>[4x]GIDPFTMTPSEDFVVTDRGGIVENSHRVHAAVVDAKGRLLYALGNPTRMTLARSAAKPAQALAILETEGVAGYGFDDADIALMCASHSSEDRHIARTRAMLSKIKAEEADLRCGGHPSLSEMVNRSWIKQDFIPTAVCSNCSGKHVGMLAGARA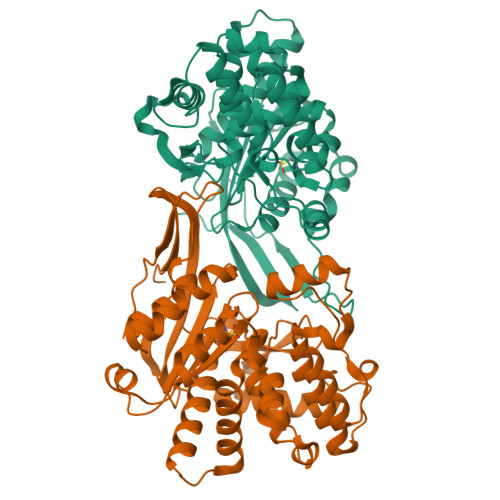IGAGTDGYHLPDHPMQGRVKRTVAELCDLDAGDVEWGTDGCNLPTPAFPLDRLGRIYAKLASAADGSDAGEGQSTRCAALAHIFRAMARHPEMVAGEGRYCTMLMRAFDGALVGKLGADASYAIGVRASDATRQLGTDGALGISVKIEDGNLEMLYAVVTELLERLGIGSPDVRSQLASFHHPQRVNTMGVTTGGVSFPFKLRGSKSNVDDPRLAAVAR>[2x]SDKKSLMPLVGIPGEIKNRLNILDFVKNDKFFTLYVRALQVLQARDQSDYSSFFQLGGIHGLPYTEWAKAQPQLHLYKANYCTHGTVLFPTWHRAYESTWEQTLWEAAGTVAQRFTTSDQAEWIQAAKDLRQPFWDWGYWPNDPDFIGLPDQVIRDKQVEITDYNGTKIEVENPILHYKFHPIEPTFEGDFAQWQTTMRYPDVQKQENIEGMIAGIKAAAPGFREWTFN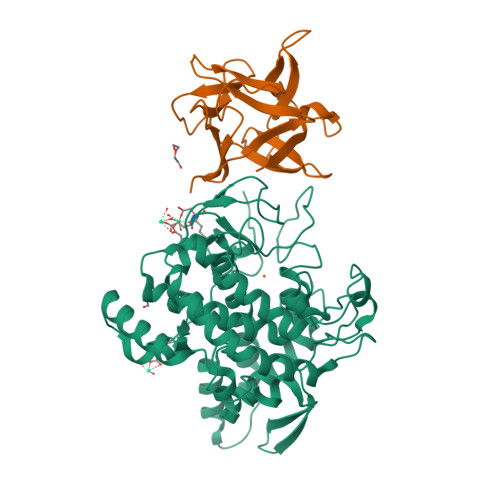MLTKNYTWELFSNHGAVVGAHANSLEMVHNTVHFLIGRDPTLDPLVPGHMGSVPHAAFDPIFWMHHCNVDRLLALWQTMNYDVYVSEGMNREATMGLIPGQVLTEDSPLEPFYTKNQDPWQSDDLEDWETLGFSYPDFDPVKGKSKEEKSVYINDWVHKHYG;>[2x]MAQARKIPLDLPGTRILNGANWANNSATENLATNSGTLIIFDQSTPGQDADRWLIHNYLDGYKIFNMGSNNWASVSRGNTVLGVSEFDGQTCKWSIEYSGNGEEFWIRVPREGGGGAVWTIKPASSQGPTTVFLDLLKETDPNQRIKFAV> MEKQVIQSVGFRNIKNGNGEITGFQFKVKLPYYRGVFLSQIRPGTLFVDGQKIEKDQITWTINGEEYTNQEMRGDFKTHWATTKPAVLKVKMPGGLAQGYHDLKYGFCFTSSYMPPIIQDGLDPDKESMVYMPEFGHHVNERRLLIVKLAAALEHHHH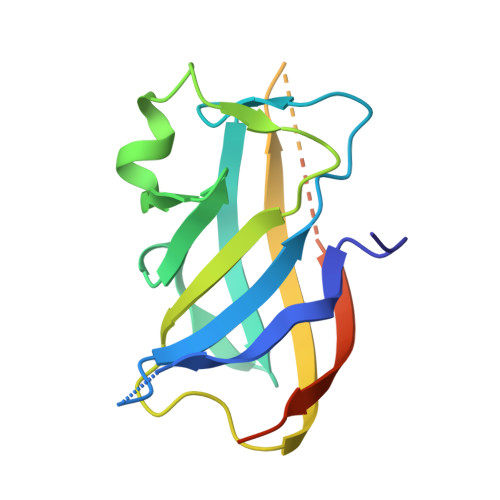HH> HLPLIAITRNPVFPRFIKIIEVKNKKLVELLRRKVRLAQPYVGVFLKRDDSNESDVVESLDEIYHTGTFAQIHEMQDLGDKLRMIVMGHRRVHISRQLEVEPEEPEAENKHKPRRKSKRGKKEAEDELSARHPAELAMEPTPELPAEVLMVEVENVVHEDFQVTEEVKALTAEI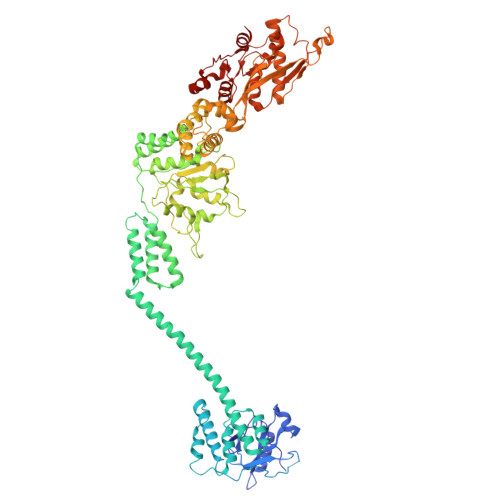VKTIRDIIALNPLYRESVLQMMQAGQRVVDNPIYLSDMGAALTGAESHELQDVLEETNIPKRLYKALSLLKKEFELSKLQQRLGREVEEKIKQTHRKYLLQEQLKIIKKELGLEKDDKDAIEEKFRERLKELVVPKHVMDVVDEELSKLGLLDNHSSEFNVTRNYLDWLTSIPWGKYSNENLDLARAQAVLEEDHYGMEDVKKRILEFIAVSQLRGSTQGKILCFYGPPGVGKTSIARSIARALNREYFRFSVGGMTDVAEIKGHRRTYVGAMPGKIIQCLKKTKTENPLILIDEVDKIGRGYQGDPSSALLELLDPEQNANFLDHYLDVPVDLSKVLFICTANVTDTIPEPLRDRMEMINVSGYVAQEKLAIAERYLVPQARALCGLDESKAKLSSDVLTLLIKQYCRESGVRNLQKQVEKVLRKSAYKIVSGEAESVEVTPENLQDFVGKPVFTVERMYDVTPPGVVMGLAWTAMGGSTLFVETSLRRPQDKDAKGDKDGSLEVTGQLGEVMKESARIAYTFARAFLMQHAPANDYLVTSHIHLHVPEGATPKDGPSAGCTIVTALLSLAMGRPVRQNLAMTGEVSLTGKILPVGGIKEKTIAAKRAGVTCIVLPAENKKDFYDLAAFITEGLEVHFVEHYREIFDIAFP Dipeptidyl peptidase III (DPP3) is a ubiquitously expressed Zn‐dependent protease, which plays an important role in regulating endogenous peptide hormones, such as enkephalins or angiotensins. DPP3 cleaves the first two amino acids at the N‐terminus of biologically important oligopeptides ranging from 3–10 amino acids. DPP3 has two big lobe‐like domains mostly composed of α‐helices with a smaller β‐sheet portion in the lower domain. Upon ligand binding, the lobes close encapsulating the substrate completely.

Not discouraged by the lack of precedence, we proposed for our DPP3 inhibitor design to incorporate a hydroxyethylene moiety instead of the cleavable peptide bond, as a noncleavable isostere resembling the transition state in peptide bond hydrolysis. We were fortunate to crystallize a SHE/hDPP3 (E451A‐variant) complex and determine its structure with X‐ray crystallography. The binding mode of SHE can be almost perfectly aligned with the binding mode of tynorphin in the previously obtained structure of tynorphin‐hDPP3 complex, the main differences being around the catalytic zinc‐complex. The C‐terminal part of the ligand is bound in a cation‐π complex of the indole moiety of SHE with Lys670 and Arg669 of hDPP3. Arg669 also forms a salt bridge to the carboxylate group of SHE. The equivalence to the tynorphin‐hDPP3 complex is also apparent at the N‐terminus of SHE, which is also tightly bound by the same three hydrogen bonds (Glu316, Asn394, Asn391) and the salt bridge to the Glu316. In contrast to the binding mode of tynorphin, the hydroxyethylene group in SHE does not interact with His568, which most probably presents a significant penalty to the enthalpy of binding. On the other hand, based on the initial rough model of binding of (S)‐hydroxyethylene type of inhibitor, the hydroxyl substituent complexes as expected to the zinc ion, which was confirmed by measurement of the bond length from the crystallographic data. The Zn−O bond was found to be 1.9 Å, which falls into the range of 1.9–2.4 Å for values typically observed for the length of Zn−O coordinating bonds in literature. Another interesting feature is a water molecule hydrogen bonded to the hydroxyethylene, which occupies the space where normally the carboxylate from Glu451 would be positioned within the active hDPP3.

> MADTQYILPNDIGVSSLDCREAFRLLSPTERLYAYHLSRAAWYGGLAVLLQTSPEAPYIYALLSRLFRAQDPDQLRQHALAEGLTEEEYQAFLVYAAGVYSNMGNYKSFGDTKFVPNLPKEKLERVILGSEAAQQHPEEVRGLWQTCGELMFSLEPRLRHLGLGKEGITTYFSGNCTMEDAKLAQDFLDSQNLSAYNTRLFKEVDGEGKPYYEVRLASVLGSEPSLDSEVTSKLKSYEFRGSPFQVTRGDYAPILQKVVEQLEKAKAYAANSHQGQMLAQYIESFTQGSIEAHKRGSRFWIQDKGPIVESYIGFIESYRDPFGSRGEFEGFVAVVNKAMSAKFERLVASAEQLLKELPWPPTFEKDKFLTPDFTSLDVLTFAGSGIPAGINIPNYDDLRQTEGFKNVSLGNVLAVAYATQREKLTFLEEDDKDLYILWKGPSFDVQVGLHALLGHGSGKLFVQDEKGAFNFDQETVINPETGEQIQSWYRSGETWDSKFSTIASSYEECRAESVGLYLCLHPQVLEIFGFEGADAEDVIYVNWLNMVRAGLLALEFYTPEAFNWRQAHMQARFVILRVLLEAGEGLVTITPTTGSDGRPDARVRLDRSKIRSVGKPALERFLRRLQVLKSTGDVAGGRALYEGYATVTDAPPECFLTLRDTVLLRKESRKLIVQPNTRLEGSDVQLLEYEASAAGLIRSFSERFPEDGPELEEILTQLATADARFWKGPSEAPSGQA> HMAQVFEECVSFINGLPRTINLPNELKLDLYKYYKQSTIGNCNIKEPSAHKYIDRKKYEAWKSVENLNREDA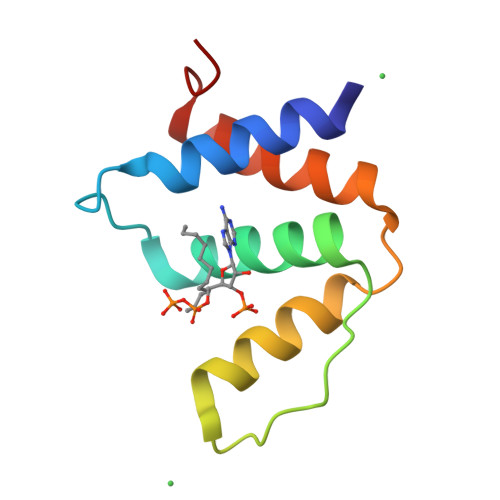QKRYVDIVSEIFPYWQD> SNAMADLLNVLKDKLSGKNVKIVLPEGEDERVLTAATQLQATDYVTPIVLGDETKVQSLAQKLNLDI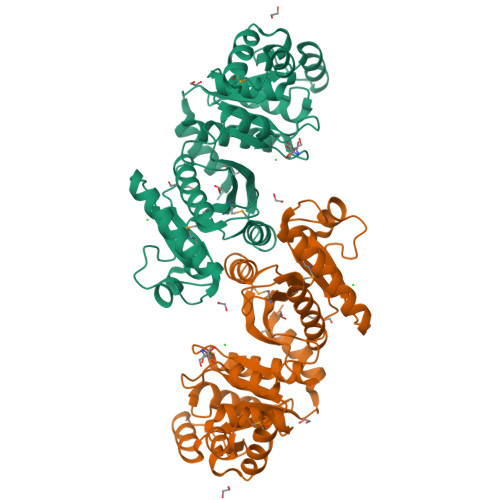SNIELINPATSELKAELVQSFVERRKGKTTEEQAQELLNNVNYFGTMLVYAGKADGLVSGAAHSTGDTVRPALQIIKTKPGVSRTSGIFFMIKGDEQYIFGDCAINPELDSQGLAEIAVESAKSALSFGMDPKVAMLSFSTKGSAKSDDVTKVQEAVKLAQQKAEEEKLEAIIDGEFQFDAAIVPGVAEKKAPGAKLQGDANVFVFPSLEAGNIGYKIAQRLGGYDAVGPVLQGLNSPVNDLSRGCSIEDVYNLSFITAAQALQ>[4x]GKAPLDEIADDSFWSDETLVKYYVNDLYSEISVDGLQLQENRSDNSVSAQRDKYRASWFKFNYDMVSASDPQDDDVWEDYYVKVRKCNRFFERIGTSTIEESEKSRLTGEVHFLRAMFYFEMVKRYGGVILLDKVLTMEDNWEIPRSSEKECYDFILEDLKK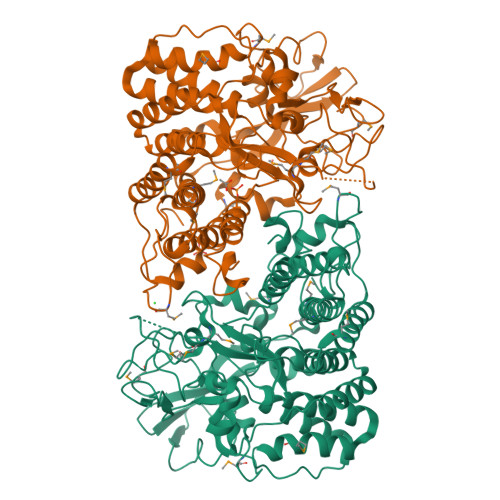ATEMLPASYGSREKGRATKGAAYALKSRVELYDKRYEDVIKSCAEVYKLGYELVDGTTPEKYRSIWWTTNKDNKEIIFDVQYKSPDVYNNMMVCNMVTYINDKYGDRGWGGLGPTQELIDAFEMADGTPATQYSQAPADQVFDINTCGIYEGREPRFYANIVFHGSQIFFNADKGAVTVDRYLMDTPDKGDGSLTGYNVWKWIDYDNYNYPYAGAGSPDFSTNWIILRYAEIYLNDAEARLETGDVEGARKAVNMIRQRVGLPDLTESDPEKLRELIRKERRIEFAFEEQRFYDVRRWKIGPETQTTLHGVRFVSPTEFKVTKTDIRTWNDRLYLTPVPHDEIVRSSVLKQNLGY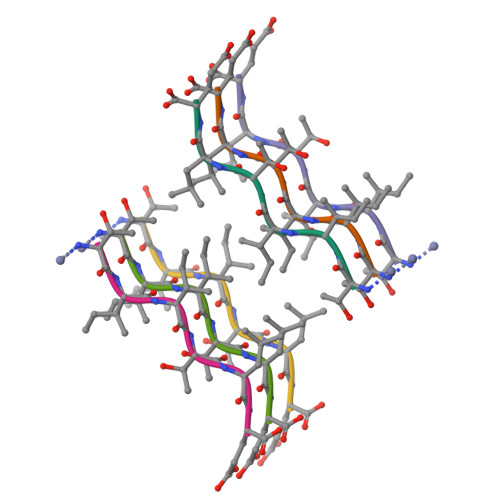> TIITLE> TGLNPN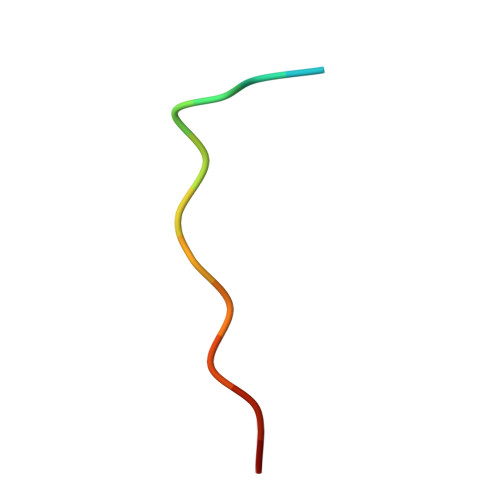AKVWQEIA> MGSSHHHHHHHHSSGLEVLFQGPGSMAAPLVTSVTETKELRGLNLIAAH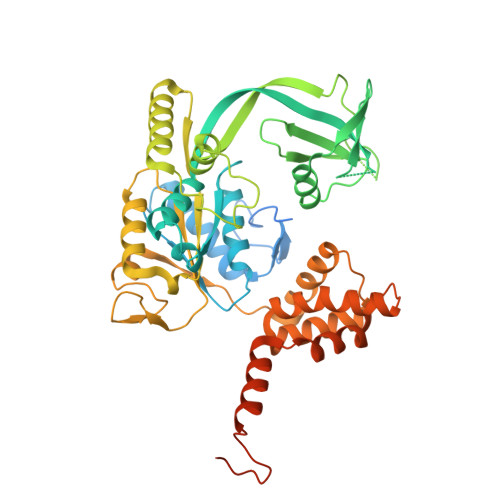SHIRGLGVDADTLEPRPSSQGLVGQEKARKAAAVVLEMIKQGKIAGRAVLIAGPPSTGKTAIAMGMAQSLGQDVPFTTLAASEIFSLEMSKTEALTQAFRKSIGVRIKEESEIMEGEVVEIQIDRSVTGGAKQGKLTIKTTDMEAIYDMGSKMIDAMTKERVMAGDIISIDKSSGKITKLGRSYARSRDYDAMGVDTKFLQCPEGELQKRKEVVHTVSLHEIDVINSRTQGFLALFSGDTGEIRSEIRDQINTKVAEWKEEGKAEIVPGVLFIDEVHMLDIECFSYINRALESDLAPIVIMASNRGVSRIRGTDYKSPHGLPLDFLDRVVIINTHPYTPDELRQILSIRAQEEEVDLTPDALALLTKIGQEAGLRYASNLITTSQLIAAKRRAKQVGVEDVQRSFKLFYDPARSVRFVQESEKRLIGNDGVVDFSYQGAAEAAAPTLPAAAPVDPVGGEKMDMS>[2x]GAMGSRADPRNQRVLLDEYSRQRGQITAGGQLLAYSVATDGRFRFLRVYPNPEVYAPVTGFYSLRYSSTALERAEDPILNGSDRRLFGRRLADFFTGRDPRGGNVDTTINPRIQQAGWDAMQQGCYGPCKGAVVALEPSTGKILALVSSPSYDPNLLASHNPEVQAQAWQRLGDNPASPLTNRAISE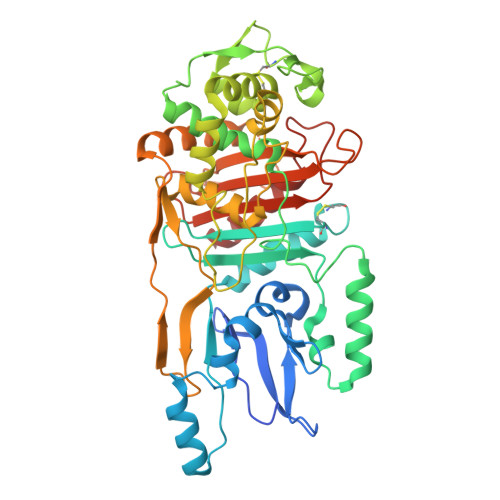TYPPGSTFKVITTAAALAAGATETEQLTAAPTIPLPGSTAQLENYGGAPCGDEPTVSLREAFVKSCNTAFVQLGIRTGADALRSMARAFGLDSPPRPTPLQVAESTVGPIPDSAALGMTSIGQKDVALTPLANAEIAATIANGGITMRPYLVGSLKGPDLANISTTVRYQQRRAVSPQVAAKLTELMVGAEKVAQQKGAIPGVQIASKTGTAEHGTDPRHTPPHAWYIAFAPAQAPKVAVAVLVENGADRLSATGGALAAPIGRAVIEAALQGEP> AMAAAPDFSSALSLRSSTATSQQNSLSTNIFASGDVSPQTPTPPQADEKTEDCLAIINKLRSENLKDLLGTLAKAEDTE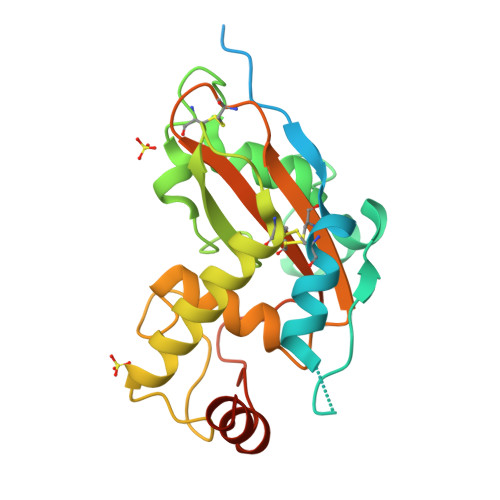VTESLKAIKIEEPASPTAPKIAVTLAGSNVDTCESGEGANAKKYPGLVIPFPHDTEFNCNALIQATYTAGLDHLKQSNFEPSTGTYDVENAPFNNVNASNVAFLLSEKSKKVSCAATKDCKAGHDVLFCYFIDPLRKEDKPFTAELYNALWGLEALEHHHHHH2-amino-L-histidine | C6 H10 N4 O2 | 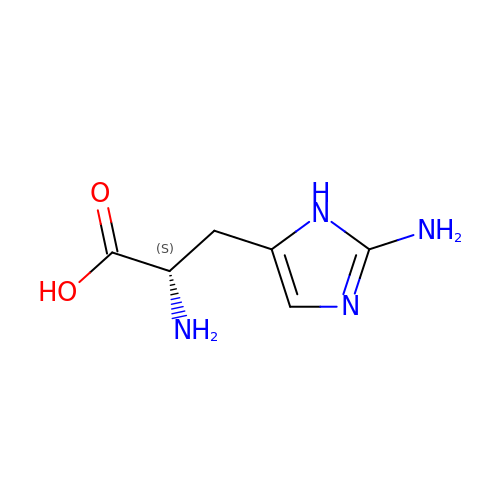UYEGXSNFZXWSDV-BYPYZUCNSA-N> MELKNLTVAIATFFASTNALALSEPSQQVTEIYQHHAHQNGNDRALPDYAPTKLLPQQPKPTLRTLSTRSAEQAANVCDVEAFTSNSSNDVLNAIKTQGASCVNALFSAESRIQEAAFESGHMYNIAKHTTDLAKAYAGGGSDELEALFLYLRAGYYAEFYNSKVSFLSWVTPAVKEAVDAFVNNANFYENSDPHGKVLSEVIITMDSAGLQHAYLPQVTQWLTRWDSQYAQNW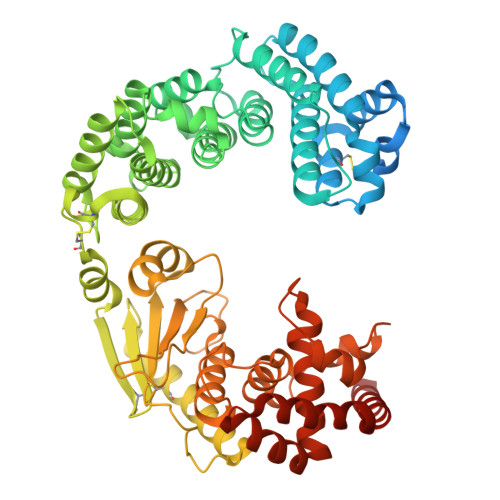YMRNAVNGVFTILFGGQWNEQFVQTIGNQTELAKALGDFALRSSAIGASDEFMAANAGRELGRLTKYSGSASSTVKSKLTEIFAQYEMYGRGDAIWLGAADTVSYYADCSDYGICNFESQLKGLVLSQSYTCSPTIRILSQNMTQDQHVAACSKMGYEEGYFHTSLETGRQPVADDYNTQLQVNIFDSSDDYGKYAGPIFNISTNNGGMYLEGDPATPGNIPNFVAYEAPYANPDHFVWNLEHEYVHYLDGRFDLYGGFGHPTERIVWWSEGIAEYVSKENDNQAAIDTIKDGSTFTLSEIFETSYDGFDVDRIYRWGYLAVRFMFERHKDDVNQMLIETRQGNWANYKATINQWAILYQSEFEQWQQALVLEHHHHHH>[2x]GLGYGSWEIDPKDLTFLKELGTGQFGVVKYGKWRGQYDVAIKMIKEGSMSEDEFIEEAKVMMNLSHEKLVQLYGVCTKQRPIFIITEYMANGCLLNYLREMRHRFQTQQLLEMCKDVCEAMEYLESKQFLHRDLAARNCLVNDQGVVKVSDFGLSRYVLDDEYTSSVGSKFPVRWSPPEVLMYSKFSSKSDIWAFGVLMWEIYSLGKMPYERFTNSETAE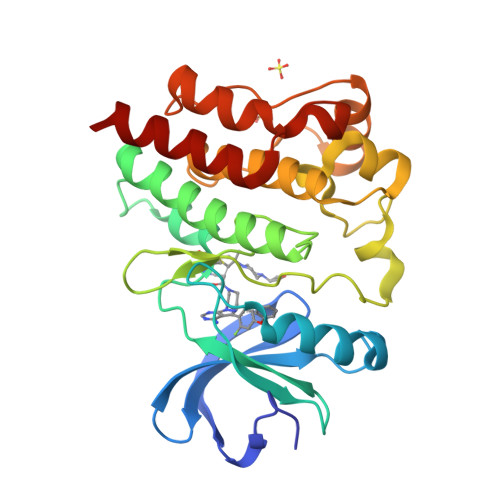HIAQGLRLYRPHLASEKVYTIMYSCWHEKADERPTFKILLSNILDVMDEES> MAQILPIRFQEHLQLQNLGINPANIGFSTLTMESDKFICIREKVGEQAQVVIIDMNDPSNPIRRPISADSAIMNPASKVIALKAGKTLQIFNIEMKSKMKAHTMTDDVTFWKWISLNTVALVTDNAVYHWSMEGESQPVKMFDRHSSLAGCQIINYRTDAKQKWLLLTGISAQQNRVVGAMQLYSVDRKVSQPIEGHAASFAQFKMEGNAEESTLFCFAVRGQAGGKLHIIEVGTPPTGNQPFPKKAVDVFFPPEAQNDFPVAMQISEKHDVVF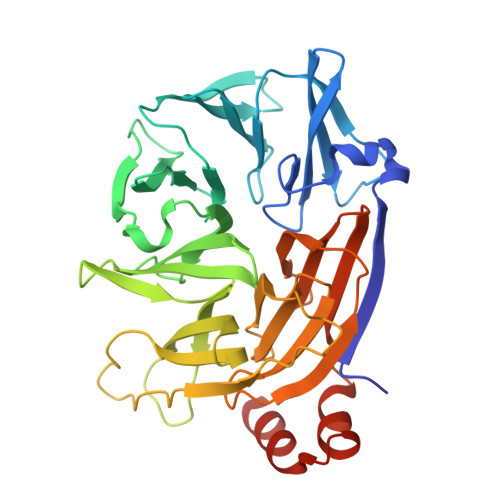LITKYGYIHLYDLETGTCIYMNRISGETIFVTAPHEATAGIIGVNRKGQVLSVCVEEENIIPYITNVLQNPDLALRMAVRNNLAGAEEL> S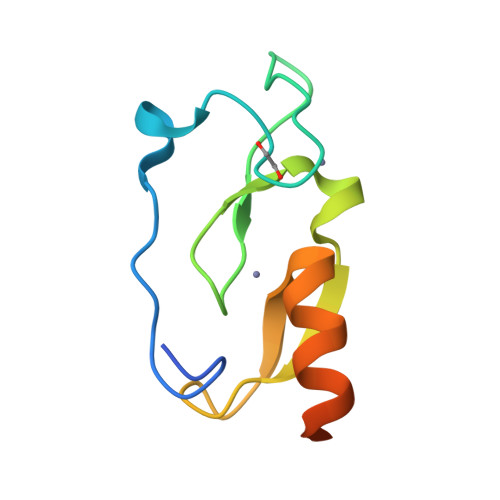MEGLVLGQKQPTWVPDSEAPNCMNCQVKFTFTKRRHHCRACGKVFCGVCCNRKCKLQYLEKEARVCVVCYETISKAQAFERMMSPTGSN5'-deoxy-5'-fluorothymidine | C10 H13 F N2 O4 | 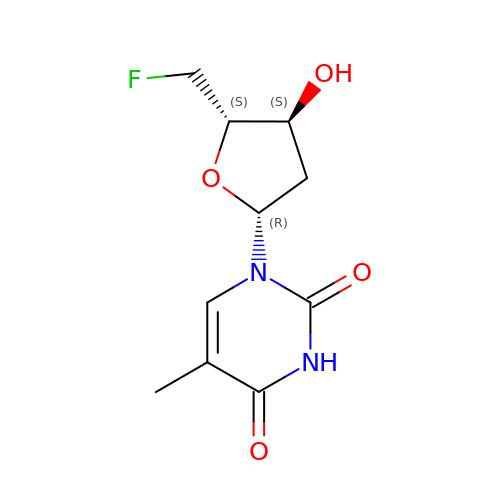MYWVPKQWFIVGJZ-XLPZGREQSA-N> MSQYLKPFELTLRCLGPVFIGSGEKRTPKEYVASTSMVYFPDMERLYADVAAQGKSESFEEFMMNTGKAQPDERFNEWIAENGVKVSPKNHGGYGVKIGSIVPGRAHRGRDGQMIQEQRQLNDIHSFIKDVLGNPYVPGSSVKGMLRSIYLQSLVHQRTAQPVRVPGHQTREHRQYGERFERKELRKSGRPNTRPQDAVNDLFQAIRVTDSPGLRTSDLLICQKMDVNVHGKPDGLPLFRECLAPGTSISLRVVVDTSPTARGGWPAGERFLETLSDTVAFVNKARYAEYAAKYWDDDPQFGPIV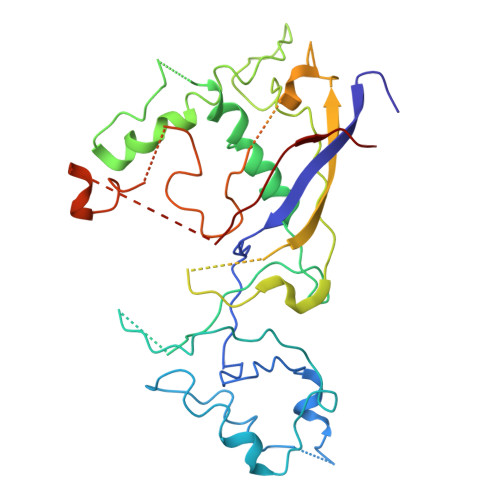YLGGGAGYRSKTFVTQQDDMAKVLDAQFPKIKHVAKTRDLGVSPLVLKLTKIGDKYYEMGQCELSIRRAE>TIEKPKISVAFIALGNFCRSPMAEAIFKHEVEKANLENRFNKIDSFG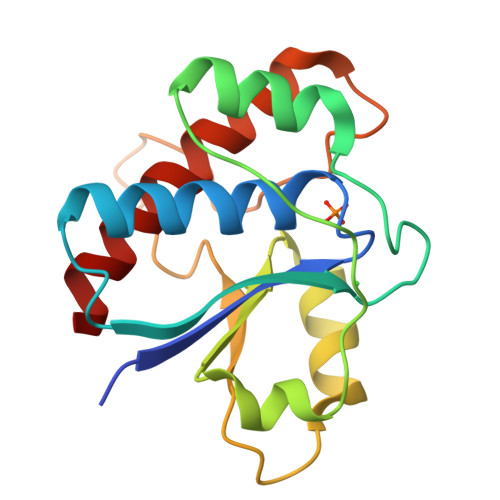TSNYHVGESPDHRTVSICKQHGVKINHKGKQIKTKHFDEYDYIIGMDESNINNLKKIQPEGSKAKVCLFGDWNTNDGTVQTIIEDPWYGDIQDFEYNFKQITYFSKQFLKKEL[2x]>ESAALVAFSTSSYSCGRKKKVNPYEEVDQEKYSNLVQSVLSSRGVAQTPGSVEEDALLCGPVSKHKLPNQGEDRRVPQNWFPIFNPERSDKPNASDPSVPLKIPLQRNVIPSVTRVLQQTMTKQQVFLLERWKQR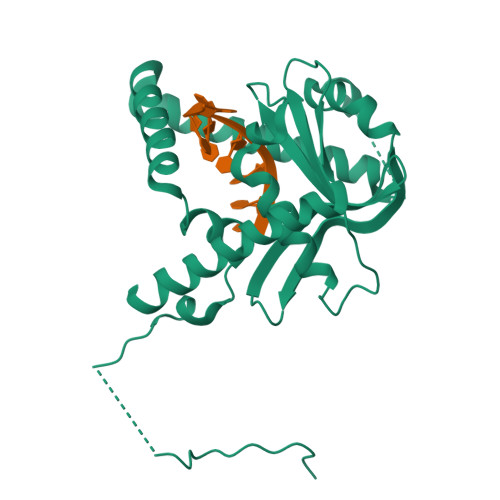MILELGEDGFKEYTSNVFLQGKRFHEALESILSPQETLKERDENLLKSGYIESVQHILKDVSGVRALESAVQHETLNYIGLLDCVAEYQGKLCVIDWKTSEKPKPFIQSTFDNPLQVVAYMGAMNHDTNYSFQVQCGLIVVAYKDGSPAHPHFMDAELCSQYWTKWLLRLEEYTEKKKNQNIQKPEYSE[4x]>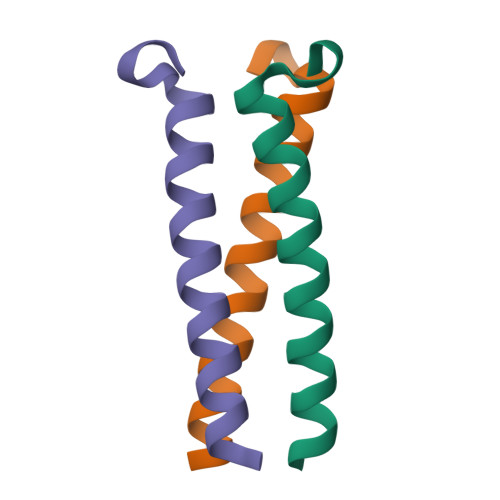XEVEALEKKVAALELKVQALEKKVEALEHGWDGR[2x]> MGHHHHHHVDLIAKKRDGYELSKEEIDFIIRGYTNG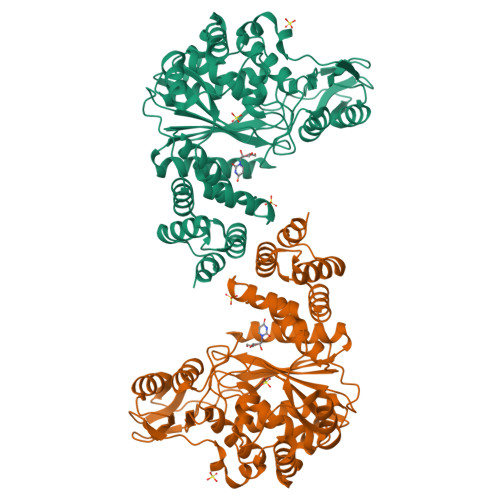DIPDYQMSAFAMAVFFRGMTEEETAALTMAMVRSGDVIDLSKIEGMKVDKHSTGGVGDTTTLVLGPLVASVGVPVAKMSGRGLGHTGGTIDKLESVPGFHVEIDNEQFIELVNKNKIAIIGQTGNLTPADKKLYALRDVTATVDSIPLIASSIMSKKIAAGADAIVLDVKTGAGAFMKDFAGAKRLATAMVEIGKRVGRKTMAVISDMSQPLGYAVGNALEVKEAIDTLKGKGPEDLQELCLTLGSYMVYLAEKASSLEEARALLEASIREGKALETFKVFLSAQGGDASVVDDPTKLPQAKYRWELEAPEDGYVAEIVADEVGTAAMLLGAGRATKEATIDLSVGLVLHKKVGDAVKKGESLVTIYSNTENIEEVKQKLAKSIRLSSIPVAKPTLIYETIS> MGSDKIHHHHHHENLYFQGMTMADETIILNVLGQYTRAHDRRDPDAMAALFAPEATIEIVDAVGGASRSISRLEGRDAIRVAVRQMMAPHGYRAWSQNVVNAPIIVIEGDHAVLDAQFMVFSILAAEVPDG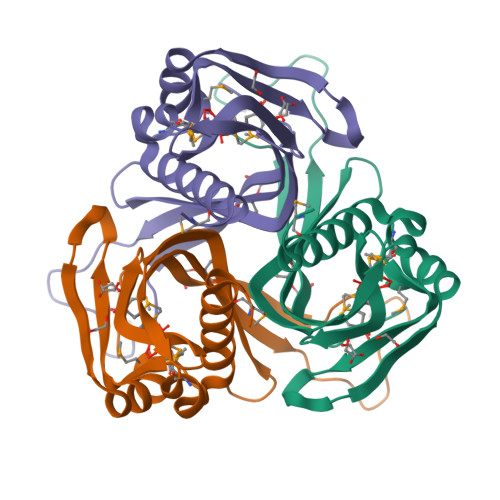GWPTGTFGAQGRIVPIEAGQYRLTLRTVADGWVISAMRIEHRLPMAFG(2R)-2-[(R)-{[(6S)-6-amino-6-carboxyhexanoyl]amino}(carboxy)methyl]-5-methyl-3,6-dihydro-2H-1,3-thiazine-4-carboxylic acid | C15 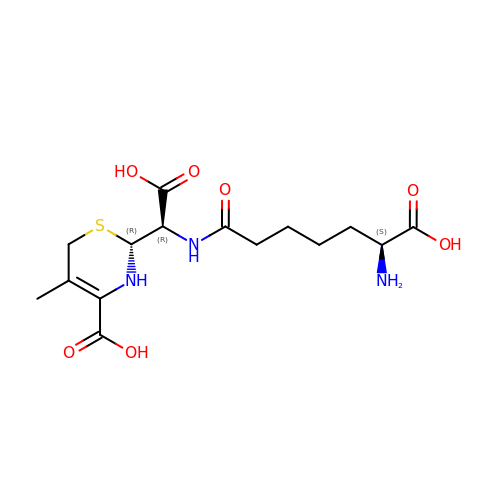H23 N3 O7 S | HJUSKFHSSKMVMT-KPXOXKRLSA-N>[2x]GGSDGLQDVTIMNQDQEQIIFAFPPVLGYGLMYQNLSSRLPSYKLCAFDFI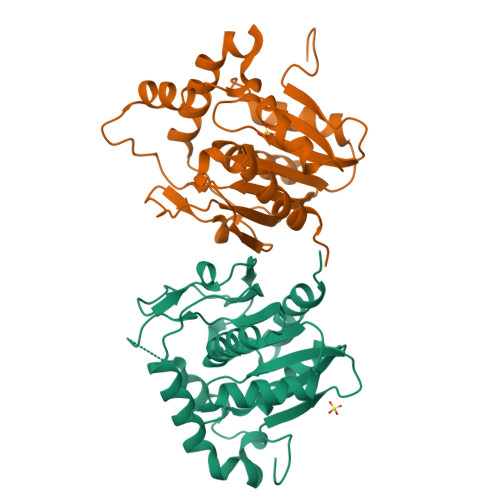EEEDRLDRYADLIQKLQPEGPLTLFGYSAGCSLAFEAAKKLEGQGRIVQRIIMVDSYKKQGVSDLDGRTVESDVEALMNVNRDNEALNSEAVKHGLKQKTHAFYSYYVNLISTGQVKADIDLLTSGADFDIPEWLASWEEATTGAYRMKRGFGTHAEMLQGETLDRNAGILLEFLNTQT>[2x]MKIAIVGVSGAVGQEFLRVLSQRDFPIDGLYLFGSSRSAGSVYSFKGKEYVVRELKDNDDFKGIDIAFCSAGGDTSIAFADTITRHGTLMIDNSSAFRMQEDVPLVVP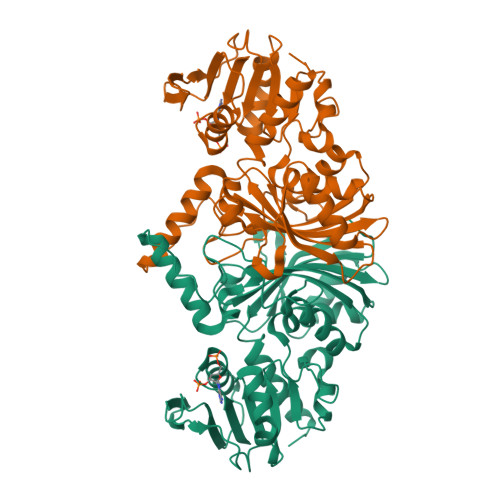EVNGDDALVHPRNIISNPNCTTIQMVVALKPIEDLSHIRRVHVATYQAASGAGALGMAELVQQVEELARGEKPTVDKFAYQLMYNLIPQIDVFTDNDYTKEEMKMYRETKRIMHSDVMVSATCVRVPVMRAHSEAIWVETERPIAPEEARAAFAKAPGVLLCDEPSEKQYPMPLFGTEQDPVIVGRIRQDLANPNGLVFWCVSDQIRKGAALNAVQIAEYLIAKGHFAR>MLSRALCSRNVPMSLKALNRPGSAGKLPMQLMKYASAVAPISHEGTLVRISQVKKLSELQLHFNDSHLGESELAAKVLGKLRKLEAEVLARNQAFNEAHPLVFDPKRAFNDEIFLCCSLCCIIFLIFLFNQYEEFAHELSFDIREQFGLGFYMLLGLHGSHVIFGTIMLALLTLWGAQGSVGPQSHALRFTSLYVHLVDLVFIILVLAIYSANASPELYGGIVPNILEARTFVSVDAAGNPQIKEF[2x];>[2x]MMQRIPFKKPNQIRGYFTRVHKYNHVPVPFILNVGMSISIVTSFVYFTYTSLWVRPEYDRVVDPSKAYVNPVWVDYWLKLRDEKRIQGALERSILEEEPEKAAEKILEWARTSAQNKILEDLKLLKPALSPATIAQFEK;>[2x]MSTVLSILGKRFQRSALTPKMNPFIRIRCQGPIEEFQRGFIGEFHAFALPGACMLVASCLGTFHIIRCLVVNPELSLAKVIPEILQPFTNPNAQLKAADGKDDDDSQVPKQWGMWGRHPNYGVLHVPFLDALNKEALARGKDGVNMGAEYNLVFTKSMADQVVDLILDDVQKRV;>[2x]MPSSMAWTIGWGFYAAWIMKETWNLRSSSVGWTPITLMEAYKTKERYLRSKAMMERYNSELEAVDDSNITEEDAKKFELEKATPSISIWEQFRSNPYWKEVEEEISTDVRKTMLEKHPDYALLLEAVKKSGYSKLWHLPGPWMNEHYNDGLHGRFLGWTPKAAHH;>[2x]VFPSITKPLGLFKNLPRQHRAARDASIWLAILTAGPFGIFIAFKYYADWYDKKLLMEYYKDSIVYGETYGKGKYV;>MLRQVVRRSNPLRMQVRGSAWNFQELMESRIPDYKGRPNRSGAELEQVKAALPKIEFMTSYEFDVLTKTRSNLTKEYSYQRDMRLKVTELMLDEAPHELEGLAVEGDAALKQLAELKALQTLTEYAGDLLEGQNQIVQRVNDFVDSNPVYLLDQPLREEARWNLLPEMDHKTRSLVRTELRDWLPAEYRQTRAVDLQQVAAFSPPVKADMFRAIEARAKDAEAEIRSLPPAEQAGLLALVKDNVAKSKAFIDPTYDITPEAINACNDVDALRAMAHRVTEYSGDARLLAIYGKAAQLTGDTAAQAILKEAKDLVF[2x];>MLRVLTPAIARPGLRCFFKDGFRDNASLELVYRVVLKSPAVSQKLIEFYAKSLDQLSVESLSALKGTTVGIPLQPYLGDPHRVLLAYSLLPHTVETEADGNPVVETKIGDEEQKIKIIDSEVISFLAKEILGKLGLETTPQAARQYLDSLVEGAEALYAKIAPVEPSPLEKAIAEINEEIKSGTPWDTLKNRADPKELHALKFAQLPHPITKKVEGKFKYF[2x];>[2x]MMNKGRILLGTNPGDIALNSKRFTVGKFVAWACGGWGLKDWIFPSLFIGRGDGPDFDRIVKHTLQSSSAIEKVNWFDSPFACYTEWFVEHFPGFFDSRYRFEMSAKTILANKYPIKDFPVVDMRSWRSSRLFDLFEVPHPEHTFVFGGPVLLNTEAKRAERLEQEWHGKDGTFVDVHPLNVATESHTEVSVIGGIKVYNGVWQGGKDSWKRDSAKPELTAPFHSPIWYRNMFIVKNADQLVEHFGENLSDETWQEVRKEHLAFHERFHKDYSFA;>[2x]MNHERPWVFLNKVTGKWGACGWQPFWKATSQSLNYIPDNFIALRTNGSWVRNLWQSSKVLDRGLNASGYPTVGTTDWVRIPLDAPLEA;>MFRRGLVLAASRSKSLLDSVHVFRPEFAQGKFRIDLDQPAKQNKLQQQIYTLTDDEREMYEDEPYIGVDHLYEAHKGSKENPVVVEAIGVHGNDVFTGCLGGCHKDAADAVAYYTIVPPNTLAVCIDCGIHFVARINEQLTFWPDGTQPWEKVDFKAVEGFLYKHYKYGSPLMI[2x];>[2x]YFFSRARMSLQLGHMRVGALWQSNANSRGLPNLLKEVMAAEPIYPYTHPGLSAKQILWNTKFNLKLEKDLISIAESAVQSQTVNKVVIPTMLTGDVNPKSPASVVAKDKYQLAKQMAEFQYKKSYFEKPWGYMFAYYCDEDRARLCGGIGYVGHHGGGDAEILSYTEYVSTVVYPTIFYMAITFVVSLFLMYYYIYGTFFSSTRNRFD;>MSTNKNVFFPPALHLKENSIFQYKFKNLAVRHDAARLGIILAGPTLFYWFTVYYFKGMPNGLPPVLLNPFVNRNYRGQKRDMPWGTDCAFLDTKCHEEKDTWAKRGPFFIIA[2x];>MEGFVDKIDDNKYLGKWETILTDGRTHLPKHITFHDAAAISARWNQQYVNDSGPVYYRHWLACQQTYGAGNEDCRKLRWWAQQITHPLHLAEWDDWWKDEHYDLQIGQHWNRICGEEFEEASNLLKDLKEKREGLAAKFRDLLKTKTAEDPMGKILHEVAQLEEPSKTPVADLVEAGTLSKEAVEAAAALKIKELKALRDDATWAEVKGSLLNGVTTTCSTLKKTSKVVAELKAQAELERNKTSAVKLDIPHMRVNYEKPGLYEYDTWFGKFLPRTPQFGFAESDEE[2x];>MLSRLLHGPGSDKGHGYFHPDHGLVDSAAQNIRGPYWHAENMQFMQQTTQSGEKLPVPLTETAAQSSKLPVLSAQDGKTLQKIQLTDGSKVPKAATLVKWNPKSVHQWHSDDILRVDMTKHPEWVRTMRMFHGTVWRHRPEFRHPWFSRGSRASGIIMLVFGAVAYGEITFGKRLGGV[2x];>MQKAVVGNLLRQLSLTRPRGHGSNLYNRVHGNLPQLYVEQLYNTDEILDTVPHSSDPVHHMFPKCAAASPLGFRPYDNNKLWDAFVLWAIVYGVTTIFCVLHILKYPQIWKHLFETLTFQYTYQREIGEEYVWQYGGGGLNPAKWRFVKSPLEELGLVTEYRSDLDYPDDL[2x];>MINNIMHMINKYTLTTSHKIIGILYGYMGYIAGILGYIISMLIRMELNTQGLAIVRKVKEVTIYNNWITIHGLIMLFVFIMPVGIGFYGNYLIPMLIGTSELSMPRMNGISFWMLIVGVVIFVISNVLMSKPISSGWTLYPPLSTRDADNIGVNIDLSLLVVHVLGISSTIGSVNYITTNKYNRHVGLTFMNINIYNFSIIVTSILLIGSLPILGVAITGLLLDRNINSTIYDVIGDPVLYQHLFWFFGHPEVYVIILPVFGLTSLILTSIIHKDIFGREGMMYCIISIGVVGYFVWAHHMFTVGLDIDSRSYFSIATSIISIPTSVKMFSYINTWASGRGFRGNNSSWSFFSFLICFCFGGFTGLLLSSGSLDIMLHDTYFVVGHFHTVLSLAATFGLLIAHYFFLPIIFSYSIFESFSFYHTFLLLVGALLVFYPMHLAGLSGMARRVPEYADIFIPFMTVGFHGTFLLIFSTLTFIRSYFQFLSHINHSNYL[2x];>[2x]MRYGNREIESIILFFDQTIILYTSIINALIVGIIIIIRKWYNRKGICNQYIYHIKIEVIWTILPIIFLIVIVLHSVTVIYNLEINKGTNNKYINVIGNQWYWIYNNIESRISSLGRIILVDQPLFIKANNNTHLIISSLDVIHSFALPTLGIKVDAIPGRINNISINGLTQGLYVGYCSELCGSGHAFMPINLIVY;>MILNTNINYGGRNSRLCYLIPLMVHTIFLYLAYLIYYNINLINIYLLLIIIIFINIEWPLVIIYEYIYLTNYNIQNNLLYNIATFIFLEILLFIGFYWLYINNIIHYPNNLPYNNNIAVNLLDHLNHNNNTDICLYIILHNLLLLLYVTLILQLVHRYVQL[2x];>[2x]MGGDAHAHGGHGLHADPIFNGSKVVRSIQMMRSYHRLPVGPEPPHLKIRGAPLHPWSMYTDKGGFFFGVGTQLPRNFFPKFLATTSAIMGVTYGLVWLYNAAGPRAKTQTRKWKELESEDPRFPFQEIPEIYLPSDIDRDPNADCWRILNQVPRKEKLLVEITDPLRNFDFKVAKIKEN;>MTTPSLSSILRHTRPIFKETLRAARPTLQNALPNGFRIASESKDGDTCTVGVWIDAGSRWETEKNNGVAHFLEHMNFKGTGKRSRQDIEFGMEKMGAHLNAYTSREHTCYYVKCFKKDVPEAVDILADILLNSKRTEQDLDAERQTIVQEKEDVEARIDEVLMDHLHSAAFEGSGLGLSILGPLENIQKSITKGMIDDFVKTHYTGPRMALVGSGAVDHGQLCDLASKYFGALPTGQPKPSGFTRFLGGDKRETNQLNPLTHVAVAFQTPGISHPDAIKIKVLEQLLGSYSRDKGEAAYSCFARAIVMDFYDPKVGQFFRPNKAGHNPIHSLNAFWAPYSDVGLLGFYAIAEPGKSYGHEWENILHYAMRELIRVSRNISEEEFERAKNQLKLQTMLQLDGTTNIADDIGRQVLSFGARVPLASFFEQLDAISREDLIRVAHEYFYDKDPVVAVIGDTDNVPEYDALRAVTYSVDLGRA[2x];>[2x]MKSVVRSKGTQALFRRFSSALGDSINPNQVGVGDNVIRVNGRLFEVDKVQEKGLKTSVLDNGTKVITLDNGGSVAQLTFLYKDGPVYENIFNAGISSFMKHALTKDGLTSSEYITKTFLQKAGIIVHEPTVVNKSAIAFTVEGFRDTLAQPAVADKFWQSLLFPRFSPENVKEVKRLVELESKETKRDSPFAYLQDILHKTAFKGSPLGHTSFVPAYNLGYIDSNKLFDRWDAHYGFGNIAVIATNIEHEAVLAAITDSAWVARAHNKVGGVAAPASKYSGGEGYDVVHRAKEFDDQFTDVYSTYTAYAFKAPGRSNLKEHAASLVIAQALSNAVSPVLNTSFAPKRLEVFYQAYDTVGLIGLSSVQASNAQLKAFKAALSKIGTLSEADLAVHKSAALLTAYGNVESWRATQATLIDSFNTTGQPLSPLEIVSAIKAVSADTVKSVVATMLGSPATLVHHGDSPCAPTLDALQ;>[2x]MNKISLYRSYSTTILLSPAYSLGFCASIFIVIQIISGYILASNYIASTNESFNIIHNVIMRELDTGWLIRFNHINGCAFLFIVIYMHIYRSLYHNSITKTSVWIVGIIMYILICGIAFTGYSLVYGQMSLWAIVVICSLVTAIPFIGNKLLILIWGGNIVSSVTLQRIFCIHYLLPLLLILFIIIHLYNLHNVNSTGDNYFINNRYDRINFYPLLLIRDVFIGSNILIIYNIFVYYYSDLFGHPDNYVPANPLVTPSEIMPEFYLLPFYALIRAIPHKVLGIIIMVLFLLSLTNLYPIYFIRFYNNINILQRSLLLLLLLDLVIASKLCLLINHYESFYLLLILSILCVLSHHIYNTSFNFSNSISNL;>GVDSHPPALPWPHFQWFQGLDWRSVRRGKEVYEQVFAPCHSLSFIKYRHFEAFMSKEEVKNMAASFEVDDDPDEKGEARKRPGKRFDTVVQPYKNEQEARYANNGALPPDLSVITNARHGGVDYIYALLTGYGRPVPGGVQLSTTQWYNPYFHGGIIGMPPPLTDDMIEYEDGTPASVPQMAKDVTCFLEWCSNPWWDERKLLGYKTIATLAVIAVSSGYYNRFLSGLWRSRRLAFRPFNYSK[2x];>MFKQLSRMYSTSPAVANAVGGLATSQIRDLVGNPAKSGKPVVKMPPYLKPSQLRPSRGAYSDEFVRENYIKAADPEDPYNYRSRAFTYAAKIPMWAGLLAGTRVTVVYLMSQFMPSKSSLALANIEVDIGDIPEGKTVTIMWQGKPVFLRKRTDAEIEDMRAVPMDALKDPQTDEERLGEGRWAVFMAVCTHLGCVPVIDQGSYNAYFCPCHGSHYDHSGRIRKGPAPLNLEVPPFKLLDDSTLFIGNADAA[2x];>GKMAAEQVSVSELKLKFEEECAHHHCHDIVKKVEVCEESIKGKEGKNCLFQHARLWECVDHCASPKVFALLK[2x];>[2x]MNDAPILAKLGLSKVNTYYFQRRKHIFALPITIPNFPLAALGIFRSTDMFEERTLERYSRDEREKTLGKAALLLKEAKEKGNYSELVRLDPTDPRHPYYFEHPWQSALKMDTVSLTPYQQYLRWHCLTYRAMHEWDRQGLLYDDLMQPKALATDPFLEEAILRLPYNQRVERERRLSRAYDLALRREYLPDEDCIHPEDDVAYLHPYYHMVVDEHREQHENPVDVYSR;>MEGHSAYVALEQRVNTRQKGIIQRHLSPYDVDIRGNGFRQIYRLGMQKIRYFGLIGTPCLLVAGAYRGIWVFCERLEDERYWSNAL[2x];>[2x]MALEIKREWHVVPATKKFADVPTEWPAKEHERFALPYGPSEGRIVSFMRASRIRNRLLFTLNPTGYTEDTYVTKEALRRQALAESKNLWYLPERPVVADQLETIVNRSTFFVVKGHKNKGLIGIAGARHNPLVWLPTLALGGVWAWRWASAGTI;>MQTHVRRVALQALRPCLRAGLMAPKFPVRFATTAVSGELLTKTPYTRPGYAAQWTCLVVLFLKNQLLMRLFFAFVAYVVAMKVFGARFHVDHDEDATPAE[2x]

Euglena gracilis, a model organism of the eukaryotic supergroup Discoba harbouring also clinically important parasitic species, possesses diverse metabolic strategies and an atypical electron transport chain. It usually involves four protein complexes (CI-CIV) constituting the electron transport chain (ETC) and a single complex V (CV) to drive ATP synthesis. Here, we report high-resolution cryo-EM structures of Euglena’s respirasome I + III2 + IV and supercomplex III2 + IV2. Euglena gracilis is a free-living, flagellated single cell eukaryote and belongs to the phylum Euglenozoa which also harbors several important parasites including Trypanosoma brucei and Leishmania donovani.

Overall 2.81 Å and 3.06 Å cryo-EM reconstructions were obtained for Eg-SC I + III2 + IV and Eg-SC III2 + IV2 respectively, using a mixed protein sample purified from E. gracilis’s mitochondria. Altogether, Eg-SC I + III2 + IV and Eg-SC III2 + IV2 have overall MWs of ~2.6 MDa and ~1.4 MDa respectively, about 1 MDa and 500 kDa larger than their opisthokont counterparts. The divergent structures of Eg-CI with a matrix FAS domain and of Eg-CIV with an inter-membrane space (IMS) helmet domain were clearly revealed from the supercomplexes. A helmet-like domain next to the cytochrome c (cyt c) binding site is also observed in Eg-CIV, likely contributing to the specific recognition for its endogenous cyt c28,30. Notably, core subunit Eg-COX3 lacks three TMHs compared to its mammalian counterpart possibly due to the evolutionary pressure of mitochondrial genome streamlining. The leftover space is occupied by TMHs of the nuclear-encoded subunit COXEG1, which introduces additional NT and CT extensions as parts of the matrix and IMS helmet domains respectively. Functional purpose of the Eg-specific matrix domain is apparently maintaining the CIII2-CIV association solely via three matrix interactions sites (Supplementary Discussion). Among them, the Eg-specific loop and β-hairpin on the NT of CIII2’s UQCRC2/MPP-α wedge into a cleft on CIV surface, formed by the matrix parts of subunits COXEG7, COXEG9, COXEG10 and COX5C. Lack of IMM or IMS interactions sites between Eg-CIII2 and Eg-CIV creates a prominent cleft between the two complexes, a feature not observed in other eukaryotic SC III2 + IV1/29–11.>MQVKPCTPEFYQTHFQLAYRLQSRPRGLALVLSNVHFTGEKELEFRSGGDVDHSTLVTLFKLLGYDVHVLCDQTAQEMQEKLQNFAQLPAHRVTDSCIVALLSHGVEGAIYGVDGKLLQLQEVFQLFDNANCPSLQNKPKMFFIQACRGDETDRGVDQQD[2x];>GKEKLPKMRLPTRSDMI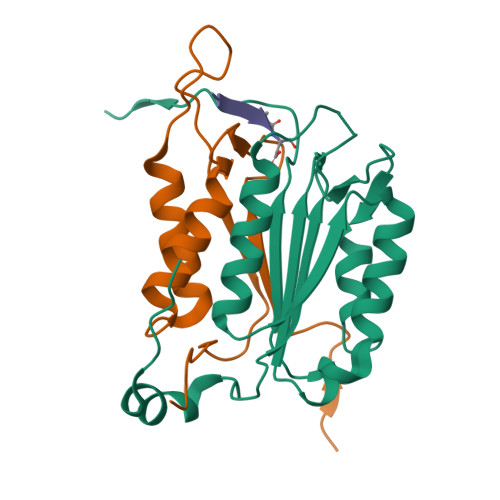CGYACLKGTAAMRNTKRGSWYIEALAQVFSERACDMHVADMLVKVNALIKDREGYAPGTEFHRCKEMSEYCSTLCRHLYLFPGHPPTLEHHHHHH[2x];>XADVAD[2x]>[2x]GSMANIAVQRIKREFKE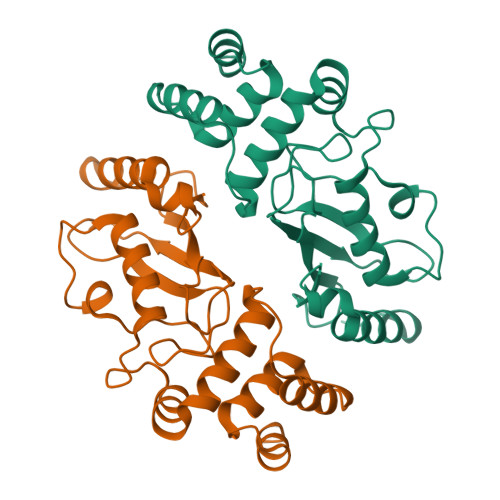VLKSEETSKNQIKVDLVDENFTELRGEIAGPPDTPYEGGRYQLEIKIPETYPFNPPKVRFITKIWHPNISSVTGAICLDILKDQWAAAMTLRTVLLSLQALLAAAEPDDPQDAVVANQYKQNPEMFKQTARLWAHVYAGAPVSSPEYTKKIENLCAMGFDRNAVIVALSSKSWDVETATELLLSN>[2x]MAHHHHHHMRQTGSFQPFFLRGKVVHGKGRGGSQLGFPTANIGLDKDVMECLQPYKNLVVYGWGTVSQVPGKERESFGPYPFAASIGFNMQFDEKTLTVE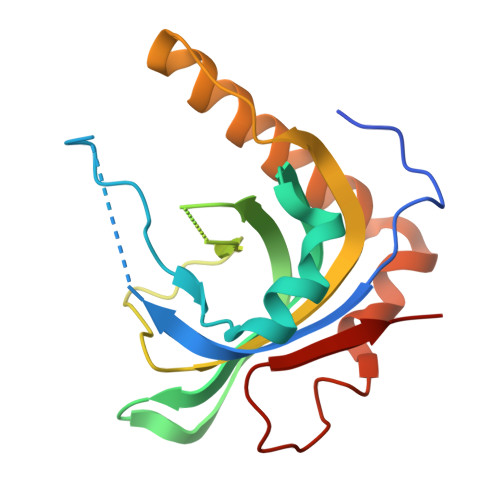PYFLHEFGWDFYGAVVKIIVLGEIRSMGSFHSLQALVDTIKSDVQFTRDMLQKPQLQEFSRHSLFESPSSTIPYFEDLPDE> MADYKDDDDKSGPDEVDASGRMGFVRQIQLLLWKNWTLRKRQKIRFVVELVWPLSLFLVLIWLRNANPLYSHHECHFPNKAMPSAGMLPWLQGIFCNVNNPCFQSPTPGESPGIVSNYNNSILARVYRDFQELLMNAPESQHLGRIWTELHILSQFMDTLRTHPERIAGRGIRIRDILKDEETLTLFLIKNIGLSDSVVYLLINSQVRPEQFAHGVPDLALKDIACSEALLERFIIFSQRRGAKTVRYALCSLSQGTLQWIEDTLYANVDFFKLFRVLPTLLDSRSQGINLRSWGGILSDMSPRIQEFIHRPSMQDLLWVTRPLMQNGGPETFTKLMGILSDLLCGYPEGGGSRVLSFNWYEDNNYKAFLGIDSTRKDPIYSYDRRTTSFCNALIQSLESNPLTKIAWRAAKPLLMGKILYTPDSPAARRILKNANSTFEELEHVRKLVKAWEEVGPQIWYFFDNSTQMNMIRDTLGNPTVKDFLNRQLGEEGITAEAILNFLYKGPRESQADDMANFDWRDIFNITDRTLRLVNQYLECLVLDKFESYNDETQLTQRALSLLEENMFWAGVVFPDMYPWTSSLPPHVKYKIRMDIDVVEKTNKIKDRYWDSGPRADPVEDFRYIWGGFAYLQDMVEQGITRSQVQAEAPVGIYLQQMPYPCFVDDSFMIILNRCFPIFMVLAWIYSVSMTVKSIVLEKELRLKETLKNQGVSNAVIWCTWFLDSFSIMSMSIFLLTIFIMHGRILHYSDPFILFLFLLAFSTATIMLCFLLSTFFSKASLAAACSGVIYFTLYLPHILCFAWQDRMTAELKKAVSLLSPVAFGFGTEYLVRFEEQGLGLQWSNIGNSPTEGDEFSFLLSMQMMLLDAAVYGLLAWYLDQVFPGDYGTPLPWYFLLQESYWLGGEGCSTREERALEKTEPLTEETEDPEHPEGIHDSFFEREHPGWVPGVCVKNLVKIFEPCGRPAVDRLNITFYENQITAFLGHNGAGKTTTLSILTGLLPPTSGTVLVGGRDIETSLDAVRQSLGMCPQHNILFHHLTVAEHMLFYAQLKGKSQEEAQLEMEAMLEDTGLHHKRNEEAQDLSGGMQRKLSVAIAFVGDAKVVILDEPTSGVDPYSRRSIWDLLLKYRSGRTIIMSTHHMDEADLLGDRIAIIAQGRLYCSGTPLFLKNCFGTGLYLTLVRKMKNIQSQRKGSEGTCSCSSKGFSTTCPAHVDDLTPEQVLDGDVNELMDVVLHHVPEAKLVECIGQELIFLLPNKNFKHRAYASLFRELEETLADLGLSSFGISDTPLEEIFLKVTEDSDSGPLFAGGAQQKRENVNPRHPCLGPREKAGQTPQDSNVCSPGAPAAHPEGQPPPEPECPGPQLNTGTQLVLQHVQALLVKRFQHTIRSHKDFLAQIVLPATFVFLALMLSIVIPPFGEYPALTLHPWIYGQQYTFFSMDEPGSEQFTVLADVLLNKPGFGNRCLKEGWLPEYPCGNSTPWKTPSVSPNITQLFQKQKWTQVNPSPSCRCSTREKLTMLPECPEGAGGLPPPQRTQRSTEILQDLTDRNISDFLVKTYPALIRSSLKSKFWVNEQRYGGISIGGKLPVVPITGEALVGFLSDLGRIMNVSGGPITREASKEIPDFLKHLETEDNIKVWFNNKGWHALVSFLNVAHNAILRASLPKDRSPEEYGITVISQPLNLTKEQLSEITVLTTSVDAVVAICVIFSMSFVPASFVLYLIQERVNKSKHLQFISGVSPTTYWVTNFLWDIMNYSVSAGLVVGIFIGFQKKAYTSPENLPALVALLLLYGWAVIPMMYPASFLFDVPSTAYVALSCANLFIGINSSAITFILELFENNRTLLRFNAVLRKLLIVFPHFCLGRGLIDLALSQAVTDVYARFGEEHSANPFHWDLIGKNLFAMVVEGVVYFLLTLLVQRHFFLSQWIAEPTKEPIVDEDDDVAEERQRIITGGNKTDILRLHELTKIYPGTSSPAVDRLCVGVRPGECFGLLGVNGAGKTTTFKMLTGDTTVTSGDATVAGKSILTNISEVHQNMGYCPQFDAIDELLTGREHLYLYARLRGVPAEEIEKVANWSIKSLGLTVYADCLAGTYSGGNKRKLSTAIALIGCPPLVLLDEPTTGMDPQARRMLWNVIVSIIREGRAVVLTSHSMEECEALCTRLAIMVKGAFRCMGTIQHLKSKFGDGYIVTMKIKSPKDDLLPDLNPVEQFFQGNFPGSVQRERHYNMLQFQVSSSSLARIFQLLLSHKDSLLIEEYSVTQTTLDQVFVNFAKQQTESHDLPLHPRAAGASRQAQDLEGSDEVDAVEGSHHHHHHHHHH

ABCA4 (also known as ABCR or the rim protein) is a retinal-specific member of the ABCA subfamily predominantly expressed in the outer segment disk membranes of photoreceptor cells, and was the first ABCA transporter that has been linked to genetic disease. Available evidence suggested that ABCA4 may act as a flippase to translocate N-retinylidene-phosphatidylethanolamine (NRPE), a reversible covalent adduct of all-trans retinal (ATR) and phosphatidylethanolamine (PE), from the luminal leaflet to the cytoplasmic leaflet of the disk membrane. Here, we show the molecular structures of human ABCA4 determined in three distinct functional states by single-particle cryo-EM to 3.3–3.4 Å. These structures delineate the conformational transitions of ABCA4 to flip NRPE and suggest a “lateral access and extrusion” mechanism for ABCA4-mediated NRPE recognition and translocation, a mechanism that might also be adopted by other ABCA transporters.

To gain structural insights into ABCA4, we first determined the structure of WT hABCA4 in the absence of NRPE and nucleotide (apo ABCA4) by single particle cryo-EM. The overall resolution of the structure is estimated to be 3.3 Å, allowing de novo model building of ABCA4 for most of the protein. In addition to the polypeptide chain, 17 sugar moieties were built into 9 glycosylation sites on ECD, which further validated the sequence assignment. The general architecture of the structure is quite similar to the torch-shaped hABCA1 structure in the nucleotide-free state, which is consistent with the 49% identity and 77% similarity between the sequences of hABCA4 and hABCA1. The discretely folded TMD1 and TMD2, each consisting of 6 TMs, contact with each other in the cytoplasmic membrane leaflet through a narrow interface between TM5 and TM11. However, other than the limited contact areas between TM5 and TM11, all the other side surfaces of TMDs are completely exposed to both leaflets of the lipid bilayer in the current conformation (defined as lateral-opening conformation), a unique structural feature among all ABC transporters and first observed in the nucleotide-free ABCA1 structure. During structural refinement, two clear phospholipid densities were observed in the cytoplasmic leaflet within the TMDs. The two phospholipids (PL1 and PL2) were found in the shallow pockets mainly enclosed by the cytoplasmic segments of TMs 1/2/5 and TMs 7/8/11, respectively. Since the presence of PE and PC molecules in our protein samples and the phospholipid head groups cannot be distinguished at current resolution, we tentatively modeled these densities as PE in our structures. The R24A/K672A/H1017A variant, designed to disrupt the PL1 binding, displayed significantly decreased ATPase activity, whereas the K1371A/Q1703A variant, designed to disrupt the PL2 binding, maintained a similar ATPase activity.>[2x]KAFPVLGIDYTHVRTPFEISLWILLACLMKIGFHVIPTISSIVPESCLLIVVGLLVGGLIKGVGETPPFLQSDVFFLFLLPPIILDAGYFLPLRQFTENLGTILIFAVVGTLWNAFFLGGLMYAVCLVGGEQINNIGLLDNLLFGSIISAVDPVAVLAVFEEIHINELLHILVFGESLLNDAVTVVLYHLFEEFANYEHVGIVDIFLGFLSFFVVALGGVLVGVVYGVIAAFTSRFTSHIRVIEPLFVFLYSYMAYLSAELFHLSGIMALIASGVVMRPYVEANISHKSHTTIKYFLKMWSSVSETLIFIFLGVSTVAGS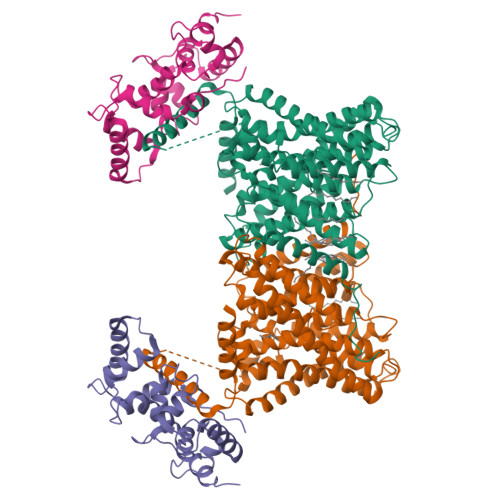HHWNWTFVISTLLFCLIARVLGVLGLTWFINKFRIVKLTPKDQFIIAYGGLRGAIAFSLGYLLDKKHFPMCDLFLTAIITVIFFTVFVQGMTIRPLVDLLAVKKKQETKRSINEEIHTQFLDHLLTGIEDICGHYGHHHWKDKLNRFNKKYV;>DEELEEIKKETGFSHSQITRLYSRFTSLDKGENGTLSREDFQRIPELAINPLGDRIINAFFPEGEDQVNFRGFMRTLAHFRPIEDNEKSKDVNGPEPLNSRSNKLHFAFRLYDLDKDEKISRDELLQVLRMMVGVNISDEQLGSIADRTIQEADQDGDSAASFTEFVKVLEKVDVEQKMSIRFLH[2x]>MEPTTEIQATEDLTLSGDHAAASADSLVVDNANDNAGQEEGFEIVLKDDETAPKQDPAKNAEFARRRIERKRQRELEQQMEAVKRGELPESLRVNPDLPPQPDINAYLSEEGLAKYDYDNSRALAAFNAANTEWLMKAQDARSNAVAEQGRKTQEFTQQSAQYVEAARKHYDAAEKLNIPDYQEK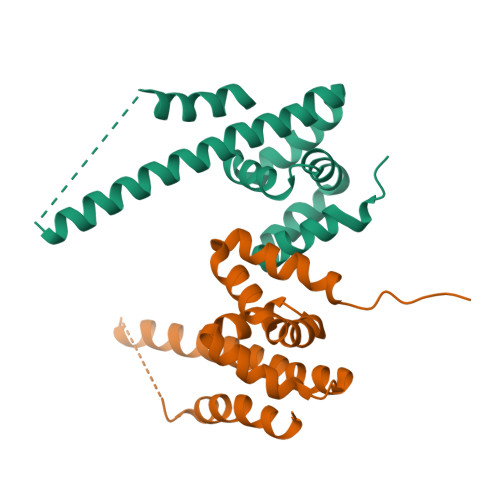EDAFMQLVPPAVGADIMRLFPEKSAALMYHLGANPEKARQLLAMDGQSALIELTRLSERLTLKPRGKQISSAPPADQPITGDVSAANKDAIRKQMDAAASKGDVETYRKLKAKLKGIR[2x]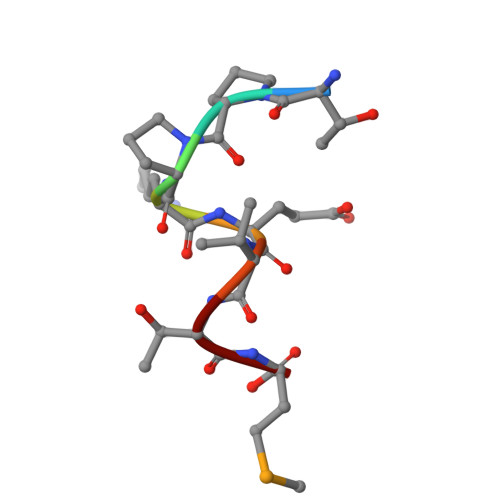> TPPKEVTM> GHMRETIREIQKVAYWLAIKGLSE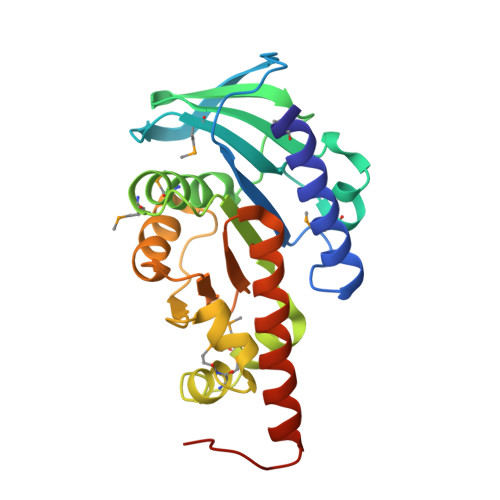ANAGNISVRLDERPEGYEVKSVNEYGFDYDGPEMYLLITATGSRMREVYEDDSKICLLHVLPGKHYEILHGNGKPTSEFPTHLMIHAKFKEMNPEKKAIVHTHPLNLLTLMNLEEFQELLPKMMKIHPEVLIFFPQGISVVEFEKPGSVELGLKTVEKSEGKDAVLWDKHGVVAFGKDVAEAYDRVEILEKAAEILLRVLSLGRNPTGVPEGWL PV, an enterovirus within the Picornaviridae family, is a positive-sense single-stranded RNA virus with a 7500 nucleotides genome enclosed within a non-enveloped icosahedral protein capsid of ~30 nm diameter. PV particles display two distinct antigenic structures, the native D antigen (D Ag) associated with mature infectious virus and the non-native C antigen (C Ag), characteristic of non-infectious particles. Virus-like particles (VLPs) that lack a viral genome represent a safer potential vaccine, although they require particle stabilization. Using our previously established genetic techniques to stabilize the structural capsid proteins, we demonstrate production of poliovirus VLPs of all three serotypes, from four different recombinant expression systems.

The rsVLPs were found in the D Ag conformation in all serotypes and expression systems, except for PV1-SC6b produced via MVA in mammalian cells. Only a C Ag particle could be reconstructed from PV1-SC6b expressed via MVA and few D Ag particles were observed in the data. In contrast, the same rsVLPs from yeast assembled significant numbers of D particles (1320 picked particles were D and 2428 were C antigenic form, a ratio of 1:1.8). The C Ag particles for PV1-SC6b (yeast and MVA) exhibited distinctive holes at their 2-fold symmetry axes compared with the D Ag particle of the same rsVLP from yeast, in line with observations of the expanded state induced in PV virions. In the case of the expanded C Ag structures observed for PV1-SC6b produced in yeast and mammalian cells, the VP1 pocket was in a collapsed state compared to that of D Ag particles; filled by sidechain residues Ile-157, Tyr-159 and Phe-237 of VP1 and consequently empty of any observable cryoEM density indicating bound lipid.

> GLGQMLESMIDNTVRETVGAATSRDALPNTEASGPTHSKEIPALTAVETGATNPLVPSDTVQTRHVVQHRSRSESSIESFFARGACVTIMTVDNPASTTNKDKLFAVWKITYKDTVQLRRKLEFFTYSRFDMELTFVVTANFTETNNGHALNQVYQIMYVPPGAPVPEKWDDYTWQTSSNPSIFYTYGTAPARISVPYVGISNAYSHFYDGFSKVPLKDQSAALGDSLYGAASLNDFGILAVRVVNDPNPTKVTSKIRVYLKPKHIRVWCPRPPRAVAYYGPGVDYKDGTLTPLSTKDLTTY;> MGAQVSSQKVGAHENSNGAYGGSTINYTTINYYRDSASNAASKQDFSQDPSKFTEPIKDVLIKTAPMLNSPNIEACGYSDRVLQLTLGNSTITAQEAANSVVAYGRWPEYLRDSEANPVDQPTEPEVAACRFYTLDTVSWTKESRGWWWKLPDALRDMGLFGQNMYYHYLGRSGYTVHVQCNASKFHQGALGVFAVPEMCLAGDSNTTTMHTSYQNANPGEKGGTFTGTFTPDNNQTSPARRFCPVDYLLGNGTLLGNAFVFPHQIINLRTNNCATLVLPYVNSLSIDSMVKHNNWGIAILPLAPLNFASESSPEIPITLTIAPMCCEFNGLRNITLPRLQ;> GLPVMNTPGSNQYLTADNFQSPCALPEFDVTPPIDIPGEVKNMMELAEIDTMIPFDLSATKKNTMEMYRVRLSDKPHTDDPILCLSLSPASDPRLSHTMLGEILNYYTHWAGSLKFTFMFCGSMMATGKLLVSYAPPGADPPKKRKEAMLGTHVIWDIGLQSSCTMVVPWISNTTYRLTIDDSFTEGGYISVFYQTRIVVPLSTPREMDILGFVSACNDFSVRLLRDTTHIEQKALAQ>RYILPSFIEHSSFGVKESNPYNKLFEERIIFLGVQVDDASANDIMAQLLVLESLDPDRDITMYINSPGGGFTSLMAIYDTMQYVRADIQTVCLGQAASAAAVLLAAGTPGKRMALPNARVLIHQPSLSGVIQGQFSDLEIQAAEIERMRTLMETTLARHTGKDAGVIRKDTDRDKILTAEEAKDYGIIDTVLEYRKLSAQTA[14x];>MRSNSQGLSLTDSVYERLLSERIIFLGSEVNDEIANRLCAQILLLAAEDASKDISLYINSPGGSISAGMAIYDTMVLAPCDIATYAMGMAASMGEFLLAAGTKGKRYALPHARILMHQPLGGVTGSAADIAIQAEQFAVIKKEMFRLNAEFTGQPIERIEADSDRDRWFTAAEALEYGFVDHIITRAHVNGEAQ[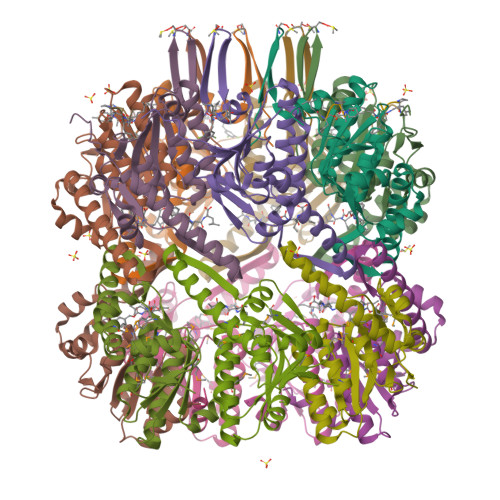14x];>[14x]FTPXAP> MSLISKEELIKLAYSIRPRENEYKTILTNLDEYNKLTTNNNENKYLQLKKLNESIDVFMNKYKTSSRNRALSNLKKDILKEVILIKNSNTSPVEKNLHFVWIGGEVSDIALEYIKQWADINAEYNIKLWYDSEAFLVNTLKKAIVESSTTEALQLLEEEIQNPQFDNMKFYKKRMEFIYDRQKRFINYYKSQINKPTVPTIDDIIKSHLVSEYNRDETVLESYRTNSLRKINSNHGIDIRANSLFTEQELLNIYSQELLNRGNLAAASDIVRLLALKNFGGVYLDVDMLPGIHSDLFKTISRPSSIGLDRWEMIKLEAIMKYKKYINNYTSENFDKLDQQLKDNFKLIIESKSEKSEIFSKLENLNVSDLEIKIAFALGSVINQALISKQGSYLTNLVIEQVKNRYQFLNQHLNPAIESDNNFTDTTKIFHDSLFNSATAENSMFLTKIAPYLQVGFMPEARSTISLSGPGAYASAYYDFINLQENTIEKTLKASDLIEFKFPENNLSQLTEQEINSLWSFDQASAKYQFEKYVRDYTGGSLSEDNGVDFNKNTALDKNYLLNNKIPSNNVEEAGSKNYVHYIIQLQGDDISYEATCNLFSKNPKNSIIIQRNMNESAKSYFLSDDGESILELNKYRIPERLKNKEKVKVTFIGHGKDEFNTSEFARLSVDSLSNEISSFLDTIKLDISPKNVEVNLLGCNMFSYDFNVEETYPGKLLLSIMDKITSTLPDVNKNSITIGANQYEVRINSEGRKELLAHSGKWINKEEAIMSDLSSKEYIFFDSIDNKLKAKSKNIPGLASISEDIKTLLLDASVSPDTKFILNNLKLNIESSIGDYIYYEKLEPVKNIIHNSIDDLIDEFNLLENVSDELYELKKLNNLDEKYLISFEDISKNNSTYSVRFINKSNGESVYVETEKEIFSKYSEHITKEISTIKNSIITDVNGNLLDNIQLDHTSQVNTLNAAFFIQSLIDYSSNKDVLNDLSTSVKVQLYAQLFSTGLNTIYDSIQLVNLISNAVNDTINVLPTITEGIPIVSTILDGINLGAAIKELLDEHDPLLKKELEAKVGVLAINMSLSIAATVASIVGIGAEVTIFLLPIAGISAGIPSLVNNELILHDKATSVVNYFNHLSESKKYGPLKTEDDKILVPIDDLVISEIDFNNNSIKLGTCNILAMEGGSGHTVTGNIDHFFSSPSISSHIPSLSIYSAIGIETENLDFSKKIMMLPNAPSRVFWWETGAVPGLRSLENDGTRLLDSIRDLYPGKFYWRFYAFFDYAITTLKPVYEDTNIKIKLDKDTRNFIMPTITTNEIRNKLSYSFDGAGGTYSLLLSSYPISTNINLSKDDLWIFNIDNEVREISIENGTIKKGKLIKDVLSKIDINKNKLIIGNQTIDFSGDIDNKDRYIFLTCELDDKISLIIEINLVAKSYSLLLSGDKNYLISNLSNTIEKINTLGLDSKNIAYNYTDESNNKYFGAISKTSQKSIIHYKKDSKNILEFYN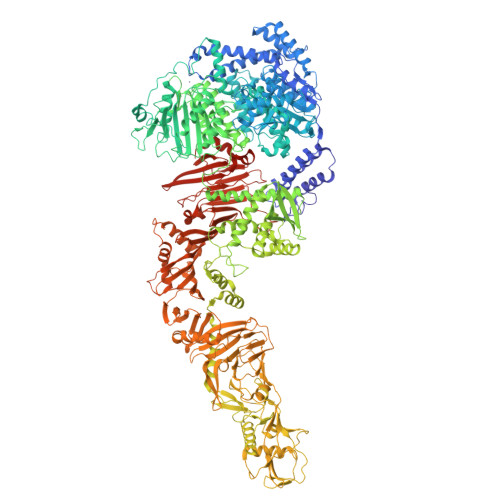DSTLEFNSKDFIAEDINVFMKDDINTITGKYYVDNNTDKSIDFSISLVSKNQVKVNGLYLNESVYSSYLDFVKNSDGHHNTSNFMNLFLDNISFWKLFGFENINFVIDKYFTLVGKTNLGYVEFICDNNKNIDIYFGEWKTSSSKSTIFSGNGRNVVVEPIYNPDTGEDISTSLDFSYEPLYGIDRYINKVLIAPDLYTSLININTNYYSNEYYPEIIVLNPNTFHKKVNINLDSSSFEYKWSTEGSDFILVRYLEESNKKILQKIRIKGILSNTQSFNKMSIDFKDIKKLSLGYIMSNFKSFNSENELDRDHLGFKIIDNKTYYYDEDSKLVKGHHHHHH>LPNITILATGGTIAGGGDSATKSNYTVGKVGVENLVNAVPQLKDIANVKGEQVVNIGSQDMNDNVWLTLAKKINTDCDKTDGFVITHGTDTMEETAYFLDLTVKCDKPVVMVGAMRPSTSMSADGPFNLYNAVVTAADKASANRGVLVVMNDTVLDGRDVTKTNTTDVATFKSVNYGPLGYIHNGKIDYQR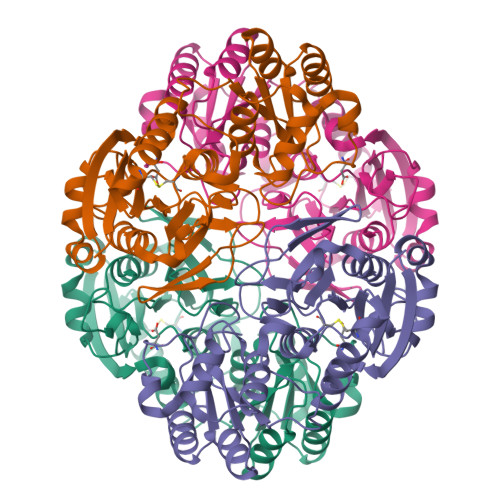TPARKHTSDTPFDVSKLNELPKVGIVYNYANASDLPAKALVDAGYDGIVSAGVGNGNLYKSVFDTLATAAKTGTAVVRSSRVPTGATTQDAEVDDAKYGFVASGTLNPQKARVLLQLALTQTKDPQQIQQIFNQY[2x]> GAMDPRTITMHKDSTGHVGFIFKNGKITSIVKDSSAARNGLLTEHNICEINGQNVIGLKDSQIADIL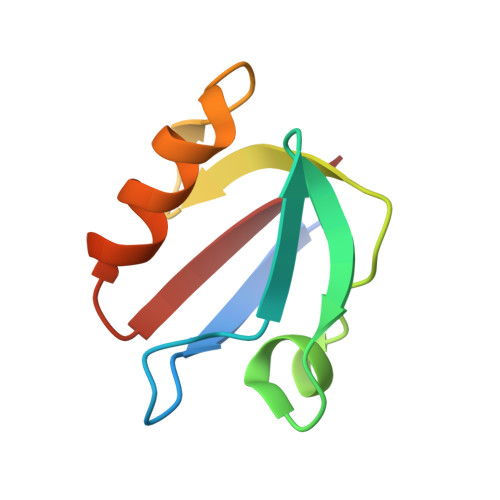STSGTVVTITIM NICOTINAMIDE-ADENINE-DINUCLEOTIDE-5-HYDROXY-4-OXONORVALINE 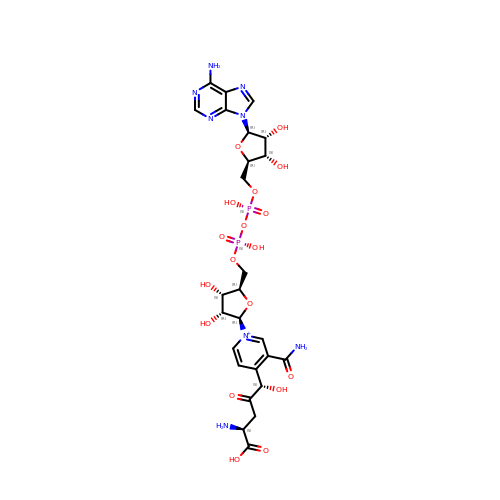| C26 H35 N8 O18 P2 | RSVNLFPFYXGAGU-GIBQRGJUSA-O>[4x]GPDSASRISPGQINQVRPKLPLLKI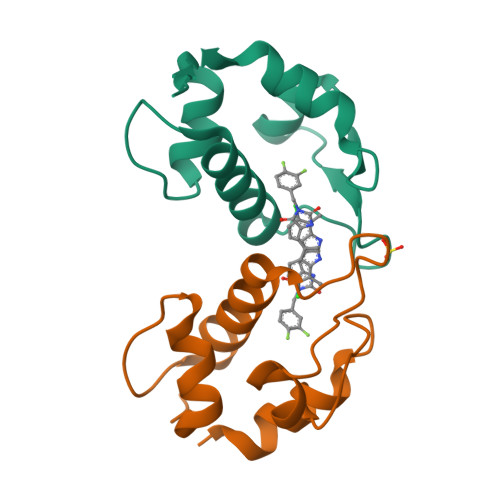LHAAGAQGEMFTVKEVMHYLGQYIMVKQLYDQQEQHMVYCGGDLLGELLGRQSFSVKDPSPLYDMLRKNLVTLAT>DDSKYQCVKLNDGHFMPVLGFGTYAPAEVPKSKALEAVKLAIEAGFHHIDSAHVYNNEEQVGLAIRSKIADGSVKREDIFYTSKLWSNSHRPELVRPALERSLKNLQLDYVDLYLIHFPVSVKPGEEVIPKDENGKILFDTVDLCATWEAMEKCKDAGLAKSIGVSNFNHRLLEMILNKPGLKYKPVCNQVECHPYFNQRKLLDFCKSKDIVLVAYSA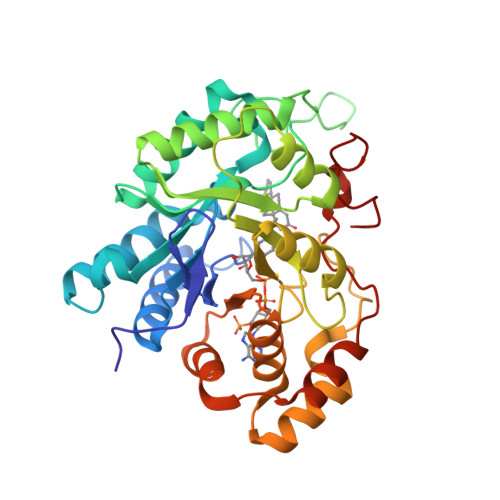LGSHREEPWVDPNSPVLLEDPVLCALAKKHKRTPALIALRYQLQRGVVVLAKSYNEQRIRQNVQVFEFQLTSEEMKAIDGLNRNVRYLTLDIFAGPPNYPFSDEY[2x]> HGSPVDICTAKPRDIPMNPMCIY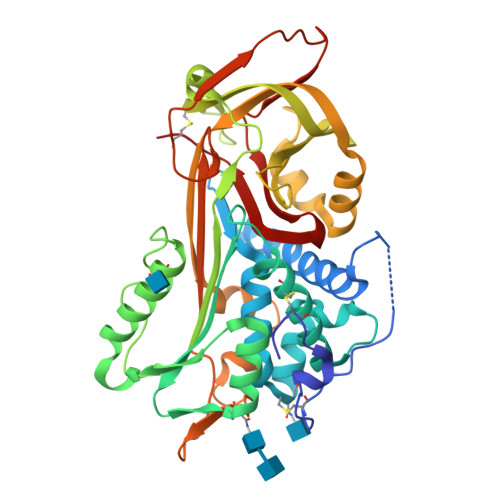RSPEKKATEDEGSEQKIPEATNRRVWELSKANSRFATTFYQHLADSKNDNDNIFLSPLSISTAFAMTKLGACNDTLQQLMEVFKFDTISEKTSDQIHFFFAKLNCRLYRKANKASKLVSANRLFGDKSLTFNETYQDISELVYGAKLQPLDFKENAEQSRAAINKWVSNKTEGRITDVIPSEAINELTVLVLVNTIYFKGLWKSKFSPENTRKELFYKADGESCSASMMYQEGKFRYRRVAEGTQVLELPFKGDDITMVLILPKPEKSLAKVEKELTPEVLQEWLDELEEMMLVVHMPRFRIEDGFSLKEQLQDMGLVDLFSPEKSKLPGIVAEGRDDLYVSDAFHKAFLEVNEEGSAAAASTAVVIAGRSLNPNRVTFKANRPFLVFIREVPLNTIIFMGRVANPCVK;> HGSPVDICTAKPRDIPMNPMCIYRSPEKKATEDEGSEQKIPEATNRRVWELSKANSRFATTFYQHLADSKNDNDNIFLSPLSISTAFAMTKLGACNDTLQQLMEVFKFDTISEKTSDQIHFFFAKLNCRLYRKANKSSKLVSANRLFGDKSLTFNETYQDISELVYGAKLQPLDFKENAEQSRAAINKWVSNKTEGRITDVIPSEAINELTVLVLVNTIYFKGLWKSKFSPENTRKELFYKADGESCSASMMYQEGKFRYRRVAEGTQVLELPFKGDDITMVLILPKPEKSLAKVEKELTPEVLQEWLDELEEMMLVVHMPRFRIEDGFSLKEQLQDMGLVDLFSPEKSKLPGIVAEGRDDLYVSDAFHKAFLEVNEEGSEAAASTAVVIAGRSLNPNRVTFKANRPFLVFIREVPLNTIIFMGRVANPCVK> DLQIGFYNTSCPTAESLVQQAVAAAFANNSGIAPGLIRMHFHDCFVRGCDASVLLDSTANNTAEKDAIPNNPSLRGFEVITAAKSAVEAACPQTVSCADILAFAARDSANLAGNITYQVPSGRRDGTVSLASEANAQIPSPLFNATQLINSFANKTLTADEMVTLSGAHS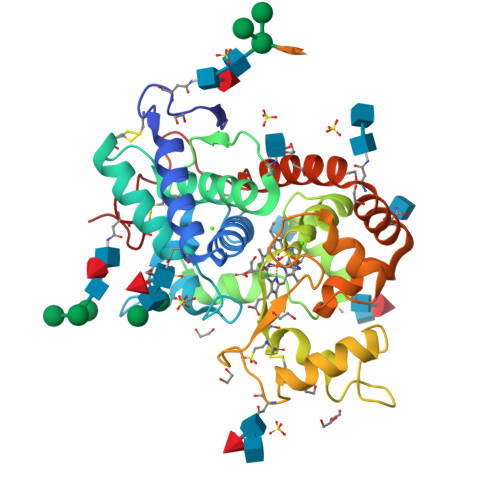IGVAHCSSFTNRLYNFNSGSGIDPTLSPSYAALLRNTCPANSTRFTPITVSLDIITPSVLDNMYYTGVQLTLGLLTSDQALVTEANLSAAVKANAMNLTAWASKFAQAMVKMGQIEVLTGTQGEIRTNCSVVNS(D) Model for RNA duplex binding and unwinding by Mss116. of short duplexes bound to D2 by excluding one RNA strand and bending the other. hydrolysis leads to core re-opening and enzyme turnover in DEAD-box proteins and perhaps other SF1 and SF2 helicases. ‘clamp’ ssRNA and form a highly stable closed-state complex.

A10-RNA + NDP-BeFx, N = A, C, G, or U. However, each base interacts differently in the ATP-binding pocket. base are missing in the structures with CDP- or UDP-BeFx. lower efficiency irrespective of the nucleotide base.

> SKLIHVPKEDNSKEVTLDSLLEEGVLDKEIHKAITRMEFPGLTPVQQKTIKPILSSEDHDVIARAKTGTGKTFAFLIPIFQHLINTKFDSQYMVKAVIVAPTRDLALQIEAEVKKIHDMNYGLKKYACVSLVGGTDFRAAMNKMNKLRPNIVIATPGRLIDVLEKYSNKFFRFVDYKVLDEADRLLEIGFRDDLETISGILNEKNSKSADNIKTLLFSATLDDKVQKLANNIMNKKECLFLDTVDKNEPEAHERIDQSVVISEKFANSIFAAVEHIKKQIKERDSNYKAIIFAPTVKFTSFLCSILKNEFKKDLPILEFHGKITQNKRTSLVKRFKKDESGILVCTDVGARGMDFPNVHEVLQIGVPSELANYIHRIGRTARSGKEGSSVLFICKDELPFVRELEDAKNIVIAKQEKYEPSEEIKSEVLEAVTEEPEDISDIVISLISSYRSCIKEYRFSERRILPEIASTYGVLLNDPQLKIPVSRRFLDKLGLSRSPIGKAMFEIRD> SVVEEHGQLSISNGELV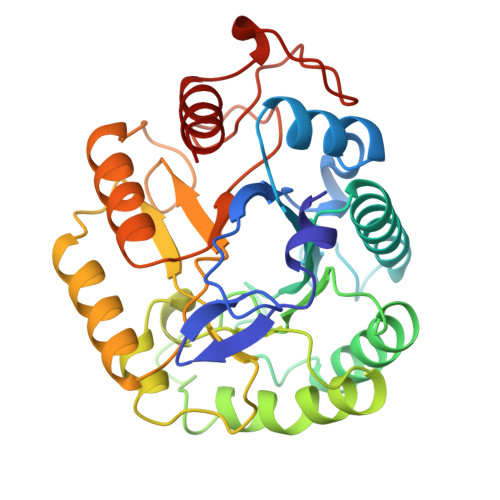NERGEQVQLKGMSSHGLQWYGQFVNYESMKWLRDDWGINVFRAAMYTSSGGYIDDPSVKEKVKEAVEAAIDLDIYVIIDWHILSDNDPNIYKEEAKDFFDEMSELYGDYPNVIYEIANEPNGSDVTWGNQIKPYAEEVIPIIRNNDPNNIIIVGTGTWSQDVHHAADNQLADPNVMYAFHFYAGTHGQNLRDQVDYALDQGAAIFVSEWGTSAATGDGGVFLDEAQVWIDFMDERNLSWANWSLTHKDESSAALMPGANPTGGWTEAELSPSGTFVREKIRES>[18x]MTIHSCLARRAVSVAASGARAFASGLGARAVAVGALQSARLLHTSSLRAAGAKISPSEMSRLLEERIAGWKTQTSTEEVGRVVSVGDGIARLFGLEGVQAGELVEFQNGMTGMALNLETDNVGVVIFGDDRSVLEGDSVKRTGRIVDVPIGPGLLGRVVDALGNPIDGKGPIPAKERRRVELKAPGIIPRKSVHEPMMTGLKCVDALVPVGRGQRELIIGDRQTGKTAVAVDAIINQKEINDSTDDESKKLYCIYVAVGQKRSTVAQIVKALEQRDAMKYTTVVAATASEAAPLQFLAPYSGCAMGEWFRDSGRHCVIIYDDLSKQATAYRQMSLLLRRPPGREAYPGDVFYLHSRLLERAAKMGDKSGGGSLTALPVIETQAGDVSAYIPTNVISITDGQIFLETELFYKGIRPAINVGLSVSRVGSAAQVKAMKQVAGTMKLELAQYREVAAFAQFGSDLDASTRQLLTRGTALTELLKQRQYSPMKNSVQVCVLYCGVKGYLDPLDPKEISRFESLFIDYINANHQDILKTIETEKELSEKTEAKLRAAVDEFVAMNEFKKK;>[6x]MQALRRGAAIPSRLLPRRDSWMSLAPFVAPNNAAAWRKLRDGAQEVQTVIERQSTPGKPQQIDWAKWESQIAHKDILNCLKTFYTNQVQILDRALGALETAKTPAPCEGAEKGWALFDAALSACAKSVEKSEELLSNGARALWVSCSNPPVWKVNTNEWLDSDQYWQAFVEKHHFYSQYQPGVVDPEAPQEVEAFKQAWHSRMGKFNDRSDTPMLYAYMNELPSWEYYDLHRSAFLEHMTYFLVRTGGDFRFFPEMPPWQWLAHMENLRFKLLSVAQSRRSQLQLANLERERALDFLPVDVEHHGEEYTQKFLQYETELFQACAARLMGHFMFLCDPFIPVQSAEALSAVTRVDNGKGKLFSLGDDVNALFYLPEQQRRDVERPTQAVQTLLGHLEATGRPFNPCYSELLHVHAEVLEERGEHWLTAPGECVSQAFLRRLRTDDPAYEVYCSYFKEMYERFAGAKEVSMEDGRKRLATIEKNAQEEAAAYGLALKTMGSAELAHKAREGAAKLEQLRKAQEKAAGKSAQTVQENKM;>[18x]MASPALQTCWRNLARLSGAQVRPSHFGAFSLGSRMSPFSSLLGARASPIATGRAGLRFLSSAAPNPGKKPASAAPPAGTNHGRITQVIGAVVDVHFDEQLPPILNSLEVQGHTNRLVLEVAQHLGENTVRTIAMDATEGLVRGQKVVDTGAPIQVPVGVETLGRIMNVIGEPVDECGPVPAKKTYSIHRAAPLFADQSTEPGLLQTGIKVVDLLAPYAKGGKIGLFGGAGVGKTVLIMELINNVANKHGGFSVFAGVGERTREGNDLYHEMMTTGVIKRKKLEDGKFDFTGSKAALVYGQMNEPPGARARVALTALSVAEYFRDEQGQDVLLFIDNIYRFTQAGSEVSALLGRIPSAVGYQPTLATDLGQLQERITTTKKGSITSVQAVYVPADDLTDPAPATTFAHLDATTVLSRQIAELGIYPAVDPLDSTSRMLAPEIVGQEHYDTARATQKLLQDYKSLQDIIAILGMDELSEEDKLVVSRARKIQRFLSQPFTVAEVFTGKPGRFVELPETIKSAQTILRGECDDLPEMAFYMCGGLEEVRSKAVKMAQEAASGK;>[6x]MNFSSSARWLAVRQSQTLGHTTRATVAAGRRVLAHSPAATEFTSFQSLHIGGDVCKLPLAVALGAAPSALGYGSAKHNQQRQYATLGSGWSFSKVQYTKYRITKPWTTDTTFDDIILSQPSKEDFAKFTKEAPLFLRFLKLVTDVEGRQEAFIQFAKRCENGLTVEKDVYVTKKELVDCLWKNGYTDTEINAFEIAFPADYKFHYPELAVLFDLTEEDCYKYCIRQRAATPEELVELKYTKPKNLVSSYGLCFLGVWFGLSNTVLSNAWFYSKTFPFGAVFYMLGSYFYRDIREKLWKEEKSLIHTAQENKNMGEESVYKQMKKYATDTKCLDYLSTFRTEVEDQIANYKVALVSQMRRQLTERLVEKLNGIQQAEKLIQGSLQDVMIREIVSSFKDLYKSRPELHDAAMQSAIQGLSGSDGAMDPVGAHFKASLQELAKVNLSTATADPMGTVVQRVAAVFQKREKEFLDTFTVKATEAQEIKTIVDKCHKGNTFDFHALSDEELRRLEQLYSTVNNRVGFETIHENSIKPVAPLSENSKGFVEFVNTQLEITKAKLRNARLTAFAHAFV;>[6x]MGGGGGGALNKLFPGYKDKIWMKVPVQWRQQMIQHWNKSYEKQVYSESVALNRTFQARNQLVLDRLKPSGAYRLPAVDYKRQLSRGTLVEGADFYLPTAQEQQRLARHFEPYSEQEQEERRKFRFQSISVYLAVALGASFVHDYFYQRRPVAWCLEKEPPHPPSYPFWFKSLFHSHDIPSVRRGYEVYRKVCATCHSMEQLHFRHLVGEVLPEKRVKQIAAEYDVTDGPNDQGEMYTRPGILGDAFPSPYPNEEAARYANGGAYPPDLSLITAARHFGPDYLMALLGGYRDPPEGVELRPGLYWNVWFPGNAIAMPPPLMDEMIDYEDGTPCNISQMSKDVVNFLTWATEPTA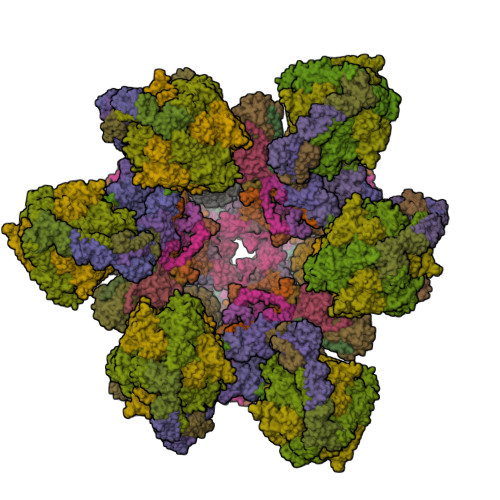DERKLYGLKCVSAIAIGTVLMTLWWRFYWAMYATRRIDFGKLKYL;>MSPVGRLFLGSKLPAQTWQSFRLQPALPQFAQKRFFSGGAAKPSWHVAREHRFGPTLPDHAYYGEHATYNYFVLFIRGMRPYLEKIFGDCASTIKNAAVAVYRPVNAFVVKHNPDLRLQFVAFASFIATHMAITKEFNDMYQRLVDITSLLELQAAQLHASEGFWDSESEQQEARLQRHAEHRNDLETTWEEALREATLARNFDVLVSYLNHGTSDGCGEHGACGHSGQNGIPPSVTWNFNAMPYGKENPDTKTFPIPDHEQPYRAFSLGFTANNLSGNWGDYIDRQDNKNALMRPARMMFTDVFIPTTK[6x];>MGEKQEEEGEEEKEGKGEGGGEGGREEEDEDGSAPVVSWLRIVEERECHEETDEAPETKIALPFSAQRSSRGFEARQVEVLVSANSAFLLSVLLASLFLSSSLPSFCPPRFLLSVLLALFKDKMAGDAPAAAAAPQQAGRTASASGVRTPGYLDLVGHSLKATSMDHGMQYSSIYWETSHRTYLPFWASLTQKFSWKIMDDQIRSFLRLPKPVTTEPFVFSSGSPYIRRYFGDADISVPVPLHAPAHFAFVPTGTVSPWEETGMETGPQGAAARGAAATAFRAVLESAWKCDIDEQIKEKLHSRAGAGAFHASGSTGGCPIPTDF[6x];>[6x]MALNRVPSRVLPFAVSGVYVHPRNACRLPAAAAVSSVPSSVSAFSSRTNFLSRSSSAVMSHPCAATARHFSFAIPPANAAALADPLPATPTPPPVFEAVSSASSGIASGTNALKNVEEVSTMERYEAAVYEESFKKPIVCLFFARFSLQSKVLLQPFLDFAASASNNATFFLIDCDRVPRAAYHARVENVPSLVVMKGDDAFRQTITDSVGVKTAGDLIQEARSALDQVLRLDQQEGGTKLQPGVSSYTHHIGVDNLNVYRKGWPVA;>[6x]MALPLLASRRLFSSFVFRGQPSTLSSNLSLVRIRGLHGGSLSPPSATLPRAVQLFSSRIAFSTAAAEDSGASQTLEGRYASALFRVAKKKNQLEKVYGDLESVRNALKDSSEFRLFVDSPAVSVQQKLDVLRQLVNRYKFDPLTGNLLTTLVENKRLPMLARVADAFDAMYRKEKGEVKCLVTSAKPLSAQQQKEIVAALQNRAGTQARLIIDYAVSPQIMGGLVVRLGEQVLDFSVATRLDRLQSQLLAPL;>[6x]MQNGVFTRENADFLVKSGADSPSSQSLLLRTSPSPLSLPRRRFIFLRSASVDLSERSSLACLAPFFCLASGVCLRSAFSLPFFARRGRPCLFFIFIFFFRVSFTANFRGKRVKMAASTIPISQWPSLLYAPPSSPANPAVEALPEMQFDDLHYPRQMLLCRGAGYSLEQCNRMAQPDARVTPENPAEKLLKEEAVAAIACLSQREGGKDEQCRYYIERMYKLANKEKQPEPGTLSKASTLACKLLGIHRPEA;>MFFSRLSLSALKAAPAREALPGLLSRQSFSSAGFSQFSSQKFFFSPSRNFSQSPLFQKHTPVHCNQRIASALVPTQQPAMTRQNPYAMQVGARYDAGVASLSAAIALMSVGGVAQGIGSLFAALVSGTARNPSIKEDLFTYTLIGMGFLEFLGIICVLMSAVLLYS[60x];>MAETREGGQSGAASILGAEAFPELLSKVPLNPQMDEDKHFNKYKWGNEPIPVNRRTGSRMNSSIYDNRNHEAVRHPWSTDARTFHPNDNPEADRINTQYSNMVSDSFPEGGFSDAPRFSSNWERLLAYHHGLYSPEKFNSTTKTADEIRLAVNDFAAKVHADDPKNACKYLMIEEFKCLQSAQARIDPQGAATKCVKWFNEWRQCAWDQEKMVKGYNYIEDRRARKHKPYIGAPDLQYS[6x];>[6x]MPSSSSEDAQGGNRFECVSNSTSPRRKNATKDEAACLQPRRSAVSGPREDVLCIRTTPQPHVRRGKSGPGRRKRMRFGRERERRDKKRGEGERKRTRFPFLRLHIEGGNANSRRPLCFPSRHSLLRNHYGSLSMAFRKVSPPKAPMSVFEARSSFLDLEQCARAAGPQRWEAECQGVRQRALQAAADVMSRECGAYGDSFFQCYRHGFRLEACQGEKATMQLLRCQRMVADRLVPL;>[6x]MGLSPAFAATAGCRLASPVANSSRFLSLLRLSRPRLNAAAPAAEAAKTLERNVPMKEILQPLWVVEPPNFLRQPVWKQFWEAQFANRSFFFFGNAWTSAAAFAFFIWWSRVFDPPPKERLDRYWLNSPKFRILSAFHNPGKRPGLKISLMTYEARYCYRGLDHPFTLNEMKDFLFKLREQYLVNKYEGIQFPFVFRQFNRVSTPGTLEVHTSPALQQQPHFHEEAAGHH;>MAAGSRFPFCTAARLSSRGTLPRLGEATFFAGAESQRSAGAFAKTLQRPFLRAPSTQLFPVGNRLGVSSARALVANAMEPRRFFAAAASAKATHALQPTGTGSVAFTRPGQGSNAQFQTSLADKTRGLLGVGFLRPTKMASFAATFLLNFRFYFMYMARTTFQAVRPLLAFSVFGEVMKLVLATMSSGLFSFLFSFVLAFEVFYFFLQCYISYTFLTMFFTVLF[6x];>MTALPPPPSANVAVSFTAAPAEPLSRGEVKAASLKLELQNIERELKDWWMSRKILRDRNIGLFNLLQHHNFAGLSVNNAKLSDSQRVMWTDLVQGKPDVEDKLSVDAREMKVDMYEKLFKQAADLENPCRMPGVAYLRCLRDTLTETQSARRSSCLNAFSSFDACRTGLLKQQSAAVENSLVRQNMADVRAKALFERRAVLLDLVEGK[6x];>MNTFFLTPAAAAARRVAVSFFARSSASGFPQHRVALRPFPSQRPAERAHNLAKSQTLRSVKAHGRQSGKKEQSTESGGRRGFRAAVGAGTGCMLAASPMLFTDYDNTASPKSELIFMAGNALGYCTERFFENEYGQSIFMFALGLAYLAMLGHEGKIHGAVWRMKHLFATNFKMVGHPRYAYALPKNPLLQDAAPTKTGSTSAKK[6x];>[6x]MSGDSVAPHQRAACEQLHSEYKQCLAKNGRTHFSACTDFHSKLRACENMLGTSYCIDEGINLMKCTKNPDPSFCAKEFVAMRECNRPQGPHLVLSSSPSSPPHYELRPEVKHLYNVDSTDLGSAVAPVRSKEQLDRVADSLKADLNLPGYGHIPYKWESLRPNPGA;>MAFAGAAAPLGVKGRSVFAGMRSFIGQRLGRLYDSFYYSQSSTKYVMVFLFPAGIFYTRFRADTKLGYHVFINEEKLYPDYSQNYFDTKWTNGRKVYLDDETTVEQLKAQIYGGKAAPENVKVACRGRVFEDADNVAMAVRAFCKRDPRLLLFQDNL[6x];>MSPPTASASVASSGSSPHMDRLLGDLKLLAAYDSAAGWQEPKAMESAFQSLSWDDADVLKALPQYLNCRGEQKRRVDFAYAALCPRPVDEKDPKQTLMSLWMKARLFSYDQKHPFVLSPFAATDKSTSAGAMTAEKPF[6x];>[6x]MVRNQRYPASPVQEIFLPEPVPFVQFDQTAPSPNSPPAPLPSPSLSQCEEQKDRYRDISSMFHRGVAGAEQVREAYNSMAKCFRRVSVAEVLESDPAFRQARNFTMDLKQAEDDQRYKQLQYGRVPSILTKYHL;>[6x]MLNFIPKRCPSVSLLFGKRPVQRIEVGQARHQLEIPVETIEKIYEGVDSRLEYHNKDYNAMKWKDFMKLKLDAYHLLEASQSETAAKSALSDLNWFSDLADIYSGQQTMAEMDVALKAQGEQKLSYPIQGKNIK;>MSWATRLLRMSSPRLGLLPLGRSVKLGGAKERVSFSQFFDSEYFWTKANVGPFFLFLFTSPFWYQGIKTVYASCRYRKLNEREIISDRYTWLHERMLEDEVERVLLEQVPAGGFDKTRPGLLLGPSTL[6x];>MPAPAASGAAAVLSKDIARSFRWMQAFAAVKGKPTAGSCAAGTAVVNPEDPTKVTLKGRYTNFSLQHIWEKYDYLQTHLLLRECMLSQVAKNPRLLDPEINAGLTPTVFMRVPPETQDPETQAKAAPQKGQAN[6x];>[6x]MATPPLQDGAPTNGGAATKPSCGARLQNFARMAIKGPSVPHSILFGVGAGCCAYAGYYLYRAMRLTFFDTESVALQSRLRYAEKQKLFHQELDRELAAGHIASLVAEYDPVATRLPFQPMQDRYRV;>MGFHFQQYIAMAGRAINPVQWTRAWRRMEGKSATEVYRDALAWTNNQFAQISRASQYRAWWWQNPLGMGLVLYGTYKAWHMIYMVRKQKKTAQLVAAAYGQGGQWLNPVPR[6x];>MPFMWRQRAYCAPVPSAFASQQPNGLGGEAGVRKPLLRSNSESLSVFSQIPDGLLGHTTSVTMGNSDIFFLPKPSNLLKIALPAFVFMPNLTIFTRAFPFYAHTSA[6x];>MSTSPGLAFANLTLLLDVPQLPAIWAVNAWRELNGLFTEMKTLAGTSDLLYPSNRYNPQNEKTNRMGRPRKYNHGEWMFGNSY[6x];>[6x]MFARAFSRFASLAAPAPQRGWNAFVLPSRHFATAAGGANPFKNQLLLTLSSPSEAIYVRTPVRSVTVPGSEGAMTMTNGHSQTVARLKAGEIIVRKGETGDEVERFFLSDGFVLFKSPEDDSGCCTAEVLGVEVVPVSMLDKESAATALQELLQQGAGATDEWTKARTLLGQELLSSVIRAAP;>MWRSSGVSFTRYASEMAALLRQCLKEPYRTQAMQRNQIHLKETVYQQGQVLTRETFNDIKKAFEAAAKHAGEK[6x];>MAGLASLSSVGALRGMRLVPAAHLLPLHSAFGQQTRNFGAGDLKIVAARMKSVKSIQKITKAMKMVAASKLRMDQRRLENGLPFATPVQKLVQRIPVDPKEKGTLAVLALSSDKGLCGGVNSFVAKQARIVIKENEMAGNAVQVYGVGDKIRSALQRTFGDRFKRIMTEVTRFPWNFGQACIIADRLMQDNPARLMVIYNHFKSAVAYDTLTLNVLTPTQAAQSAKEQLNTFEFEPEKTDVWKDLQDFYYACTVFGCMLDNIASEQSARMSAMDNASTNAGEMISSLTLRYNRARQAKITTELVEIISGANALE[6x];>MSSPCCVAIRRVARTTLESGRRQVDSKSTDVSPFFTGTQQMSLPSAGMVTKIRNFSSVKFMDQKRSGEETVYFKKEDEALLRNLLANHPEYDPKYSVDHMNAEVGSIARDITLACQKHGMKDPSAAFMKDLISIFGAHGYAKNSK[6x]DExD/H-box RNA helicases, from virus and bacteria to eukaryotes, play important roles in processes including ribosome biogenesis, RNA processing and folding, ribonucleoprotein (RNP) remodeling, RNA nuclear export, the regulation of RNA translation and transcription, and nonsense-mediated RNA decay. DExD/H-box proteins often contain accessory regulatory domains and localization modules, but their cores consist of two RecA-like domains joined by a short flexible linker. The N-terminal domain is commonly referred to as conserved domain-1, or DEAD-domain, and the C-terminal domain as conserved domain-2, or helicase domain. Both domains contribute to the binding site for RNA substrates and both contribute to ATP hydrolysis. We used X-ray crystallography to determine the structures of the DEAD-domains of DDX2A, DDX2B, DDX5, DDX10, DDX18, DDX20, DDX47, DDX52, and DDX53, as well as the helicase domains of DDX25 and DDX41.

DDX53 (CAGE) is expressed in testis and various tumors, but not in other tissues. Expression of the CAGE-gene is determined by its methylation status. The 6th residue upstream of the conserved glutamine is an aromatic residue in most DEAD-box helicases. Its side chain stacks with the nucleotide base, stabilizing it in its position. Moreover, an aromatic residue in this position is not obligatory: DDX53 features an isoleucine, with weaker van-der-Waals interactions with the adenosine ring than the base stacking interactions with the aromatic side chains. In the crystal complexes with either ADP or AMP the loop closes up, resulting in a shift in Cα-atom positions by up to 3.5 Å between the ATP- and the AMP-states, or by up to 2.5 Å between the ADP- and the AMP-state.

>[2x]MTCDDLKSGEKRLIPKPTCRFKDAFQQYPDLLKSIIRVGILKPTPIQSQAWPIILQGIDLIVVAQTGTGKTLSYLMPGFIHLDSQPISREQRNGPGMLVLTPTRELALHVEAECSKYSYKGLKSICIYGGRNRNGQIEDISKGVDIIIATPGRLNDLQMNNSVNLRSITYLVIDEADKMLDMEFEPQIRKILLDVRPDRQTVMTSATWPDTVRQLALSYLKDPMIVYV> SNMWVIGKNKAQDAKAIMVNGPQFGWYVPAYTYGIGLHGAGYDVTGNTPFAYPGIVFGHNGTISWGSTAGGGDDVDIFAEKLSAEKPGYYQHNGEWVKMLSRKETIAVKDGQPETFTVWRTLHGNVIWTDTATQTAYAKARAWDGKEVASLLAWTHQMKAKNWPEWTQQAAKQALTINWYYADVNGNIGYVHTGAYPDRQP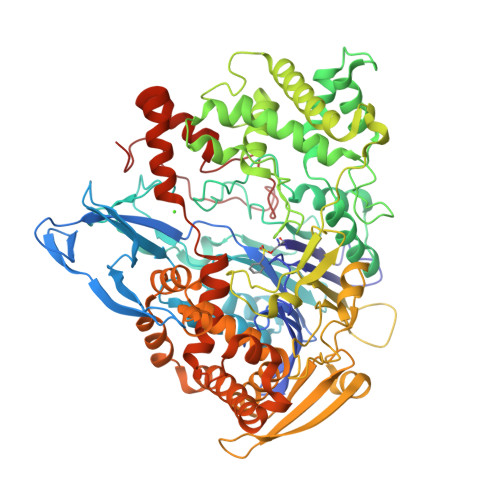GHDPRLPVPGTGKWDWKGLLSFDLNPKVYNPQSGYIANWNNSPQKDYPASDSFPFLWGGADRVTEIDTILDKQPRFTADQAWDVIRQTSRRDLNLRLFLPALKDATANLAENDPRRQLVDKLASWDGENLVNDDGKTYQQPGSAILDAWLTSMLKRTVVAAVPAPFGKWYSASGYETTPDGPTGSLNISVGAKILYEALQGDKSPIPQAVDLFGGKPQQEVILAALDDAWQTLSKRYGNDVDSWKTPAMALTWRANNFFGVPQAAAKEARPQAEYQNRGTENDMIVFSPTSGNRPVLAWDVVAPGQSGFIAPDGKKDKHYDDQLKMYESFGRKSLWLTPQDVDEHQESQEVLQVQLDQGEVKIVRDEYGMPHIYADDTYRLFYGYGYVVAQDRLFQMEMARRSTQGTVSEVLGKAFVSFDKDIRQNYWPDSIRAQIASLSAEDKSILQGYADGMNAWIDKVNASPDKLLPQQFSTFGFKPKHWEPFDVAMIFVGTMANRWSDSTSEIDNLALLTALKDKYGKQQGMAVFNQLKWLVNPSAPTTIAARESAYPLKFDLQNTQTAHHHHHH>[3x]SNAMIVGIGIDIIELNRIEKMLDGKLKFMERILTENERNVAKGLKGSRLTEFVAGRFAAKEAYSKAVGTGIGKEVSFLDIEVRNDDRGKPILITSTEHIVHLSISHSKEFAVAQVVLESSSS

The active form of ACP is produced by a post-translational modification of a conserved serine residue of apo-ACP by a 4′-phosphopantetheine (P-pant) group transferred from CoA bound to a holo-(acyl-carrier-protein) synthase (AcpS). AcpS belongs to the phosphopantetheine transferase (PPT) family of proteins, binds CoA and its derivatives and requires magnesium for activity. The AcpS trimer binds three CoA molecules and three ACP molecules. The AcpS monomer has an elongated elliptical shape and possesses an α/β fold.

The structure of AcpSBA is emphasized because of the two 3′,5′-adenosine diphosphate (3′,5′-ADP) product molecules that are found in each of the three coenzyme A (CoA) binding sites of the trimeric protein. One 3′,5′-ADP is bound as the 3′,5′-ADP part of CoA in the known structures of the CoA–AcpS and 3′,5′-ADP–AcpS binary complexes. The position of the second 3′,5′-ADP has never been described before. It is in close proximity to the first 3′,5′-­ADP and the ACP-binding site. AcpSBA only gave well diffracting crystals when the protein had the tag removed and it was pre-incubated with CoA. However, the presence of 200 mM MgCl2 in the crystallization condition appears to have been sufficient for the AcpS to hydrolyze the 10 mM CoA in the crystallization mixture even in the absence of ACP. Mg-III is also a distance of ∼5 Å from Mg-I and Mg-­II and bridges ADPI and ADPII in the AcpSBA structure. Lastly, it is important to stress the specific ADPI 5′-P–ADPII 3′-P interaction through Mg-III. Although we think that ADPII is a crystallographic artifact, the biological relevance of ADPII should be further investigated. For example, the presence of a bulky ligand that would mimic the two bound 3′,5′-ADP molecules at the interaction interface between two adjacent monomers in the AcpS trimer may prevent the binding of CoA and/or the formation of a productive CoA–AcpS–ACP complex.4-{2,4-BIS[(3-NITROBENZOYL)AMINO]PHENOXY}PHTHALIC ACID | C28 H18 N4 O11 | 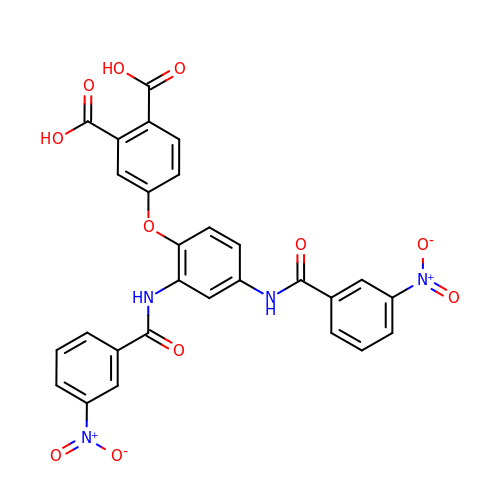VFYAZSTYKPFSFL-UHFFFAOYSA-N> MDSIQAEEWYFGKITRRE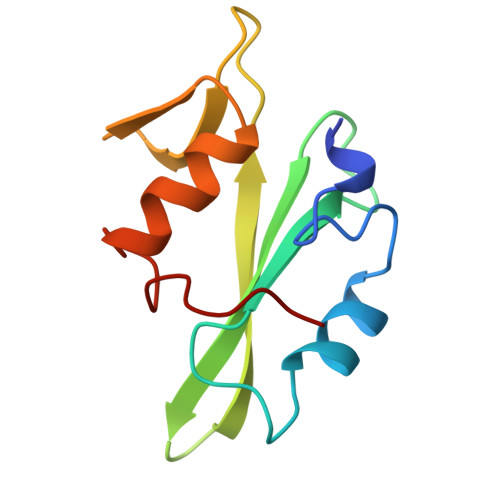SERLLLNAENPRGTFLVRESETTKGAYCLSVSDFDNAKGLNVKHYKIRKLDSGGFYITSRTQFNSLQQLVAYYSKHADGLCHRLTTVCP2-{5-[(2-{[3,5-difluoro-4-(1-methylpiperidin-4-yl)phenyl]amino}-5-methylpyrimidin-4-yl)amino]-2-fluorophenyl}-1lambda~6~,2-thiazolidine-1,1-dione | C26 H29 F3 N6 O2 S | 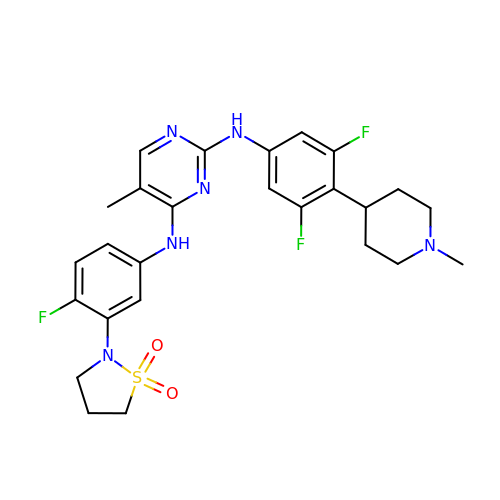YFAXWSXYQLAMER-UHFFFAOYSA-N> MGDRGPEFELGTRGSPMETLITAMEQLYTLGALDDEGLLTRLGRRMAEFPLEPMLCKMLIMSVHLGCSEEMLTIVSMLSVQNVFYRPKDKQALADQKKAKFHQTEGDHLTLLAVYNSWKNNKFSNPWCYENFIQARSLRR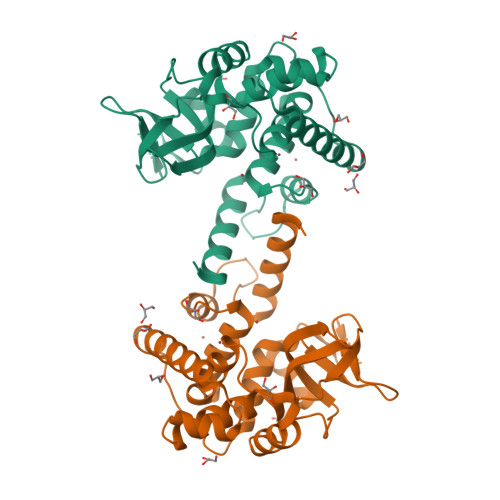AQDIRKQMLGIMDRHKLDVVSCGKSTVRVQKAICSGFFRNAAKKDPQEGYRTLIDQQVVYIHPSSALFNRQPEWVVYHELVLTTKEYMREVTTIDPRWLVEFAPAFFKVLEVDLQGDHGLSAWSHPQFEK4-(4-{[4-(4-cyano-2,6-dimethylphenoxy)pyrimidin-2-yl]amino}piperidin-1-yl)benzenesulfonamide 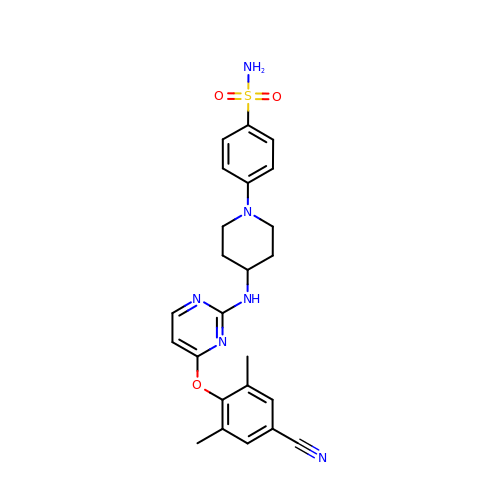| C24 H26 N6 O3 S | GZMNOTZGPCNHSP-UHFFFAOYSA-N> GAMAVNAVHLESDAFLVCMNHALSTEKEEVMGLCIGEVDTNRIVHIHSVIILRRSDKRKDRVEISPEQLSAASTEAERLAEMTGRPMRVVGWYHSHPHITVWPSHVDVRTQAMYQMMDQGFVGLIFSCFIEDKNTKTGRVLYTCFQSVQAQKGSEYERIEIPIHVVPHEAIGKVCLESAVELPRILCQEEQDTYRRIHSLTHLDPITKIHNGSVFTKNLCSQMSAISGPLLQWLEDRLEQNKQSIITLQKEKELLTQELAAL

BRCC36 is the catalytic subunit responsible for the majority of K63-Ub specific DUB activity in the cytoplasm and in the nucleus as part of two distinct macromolecular assemblies characterized by the presence of either of the MPN− pseudo DUB proteins KIAA0157 or Abraxas. The Abraxas complex (ARISC) functions in DNA repair and breast cancer suppression, while the BRCC36 isopeptidase complex (BRISC) promotes interferon dependent responses by deubiquitinating and stabilizing the type I interferon receptor, IFNAR1. BRCC36 consists of a functional metalloprotease JAMM/MPN+ domain followed by a predicted coiled coil region implicated in protein-protein interactions. KIAA0157 and Abraxas are required for the catalytic function of BRCC36 in both complexes, and enable association of two additional shared subunits (BRCC45 and MERIT40) to each holoenzyme.

To understand how KIAA0157 supports the catalytic function of BRCC36, we set out to solve an inactive-state structure of BRCC36 in isolation. Unlike CfBRCC36, which showed a propensity to aggregate at high protein concentrations, DrBRCC36 existed as a concentration dependent monomer-dimer in equilibrium and readily crystallized (see Table 1 for data collection and refinement statistics). Interestingly, DrBRCC36 adopted the analogous homodimer configuration involving the MPN domain (buried SA = 1693 Å2) displayed by the CfBRCC36-KIAA0157ΔC heterodimer (B for stereo view and combined sequence alignment), with the main exception that the CCHB helices α4 and α5 were completely disordered. While the MPN+ domains of DrBRCC36 and CfBRCC36 were highly similar (RMSD of 2.0 Å over 140 Cα atoms), notable differences in the active site region of DrBRCC36 were apparent that might account for its lack of DUB activity in comparison to CfBRCC36 complexed to KIAA0157. In particular, the E-loop of the DrBRCC36 inactive structure was partially disordered and shifted with respect to the CfBRCC36 active structure, giving rise to a 4-5 Å displacement of the catalytic glutamate (Glu30 in CfBRCC36; Glu27 in DrBRCC36). Additionally, a major portion of Ins-1 was disordered and the ordered portion (helix α2) was shifted relative to the corresponding position in CfBRCC36. Both of these structural distortions may be attributable to the loss of supporting interactions afforded by heterodimerization of CfBRCC36 with CfKIAA0157, as follows: Firstly, in the active heterodimer structure, a productive conformation of CfBRCC36 Ins-1 appears supported by direct contacts to CfBRCC36 helix α4, including between the invariant Arg53 (Ins-1) and Asp186 (α4) side chains and between the backbone carbonyl of Arg53 (Ins-1) and the invariant Glu183 (α4) side chain. The absence of the CCHB elements (specifically helix α4) in the inactive structure precluded formation of these interactions.>[2x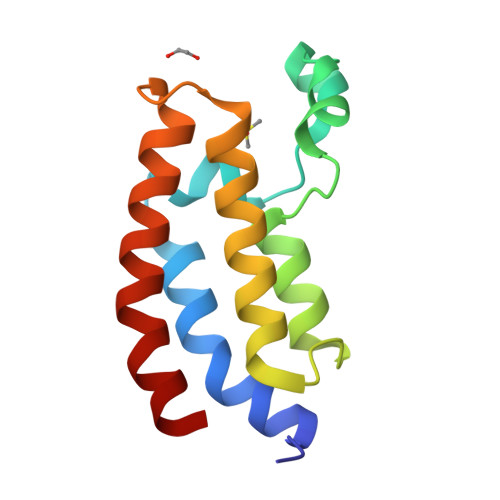]AAFKPEELRQALMPTLEALYRQDPESLPFRQPVDPQLLGIPDYFDIVKNPMDLSTIKRKLDTGQYQEPWQYVDDVWLMFNNAWLYNRKTSRVYKFCSKLAEVFEQEIDPVMQAL>[2x]MAHMERFQKVYEEVQEFLLGDAEKRFEMDVHRKGYLKSMMDTTCLGGKYNRGLCVVDVAEAMAKDTQMDAAAMERVLHDACVCGWMIEMLQAHFLVYDDIMDHSKTRRGKPCWYLHPGVTAQVAINDG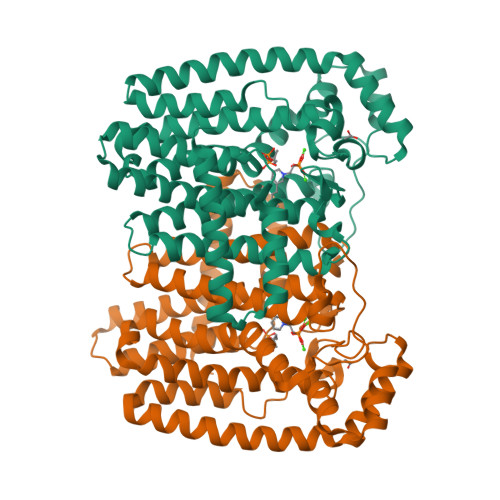LILLAWATQMALHYFADRPFLAEVLRVFHDVDLTTTIGQLYDVTSMVDSAKLDAKVAHANTTDYVEYTPFNHRRIVVYKTAYYTYWLPLVMGLLVSGTLEKVDKKATHKVAMVMGEYFQVQDDVMDCFTPPEKLGKIGTDIEDAKCSWLAVTFLTTAPAEKVAEFKANYGSTDPAAVAVIKQLYTEQNLLARFEEYEKAVVAEVEQLIAALEAQNAAFAASVKVLWSKTYKRQK>[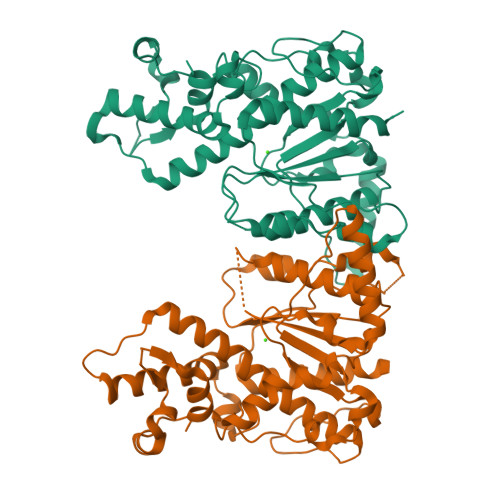2x]MPFTYSIEATRNLATTERCIQDIRNAPVRNRSTQFQLAQQNMLAYTFGEVIPGFASAGINGMDYRDVIGRPVENAVTEGTHFFRDDFRVDSNAKAKVAGDIFEIVSSAVMWNCAARWNSLMVGEGWRSQPRYSRPTLSPSPRRQVAVLNLPRSFDWVSLLVPESQEVIEEFRAGLRKDGLGLPTSTPDLAVVVLPEEFQNDEMWREEIAGLTRPNQILLSGAYQRLQGRVQPGEISLAVAFKRSLRSDRLYQPLYEANVMQLLLEGKLGAPKVEFEVHTLAPEGTNAFVTYEAASLYGLAEGRSAVHRAIRELYVPPTAADLARRFFAFLNERMELVNGENLYFQSHHHHHH>[2x]GSANDSPAKSLVDIDLSSLRDPAGIFELVEVVGNGTYGQVYKGRHVKTGQLAAIKVMDVTEDEEEEIKLEINMLKKYSHHRNIATYYGAFIKKSPPGHDDQLWLVMEFCGAGSITDLVKNTKGNTLKEDWIAYISREILRGLAHLHIHHVIHRDIKGQNVLLTENAEVKLVDFGVSAQLDREVGRRNTFIGTPYWMAPEVIACDENPDAT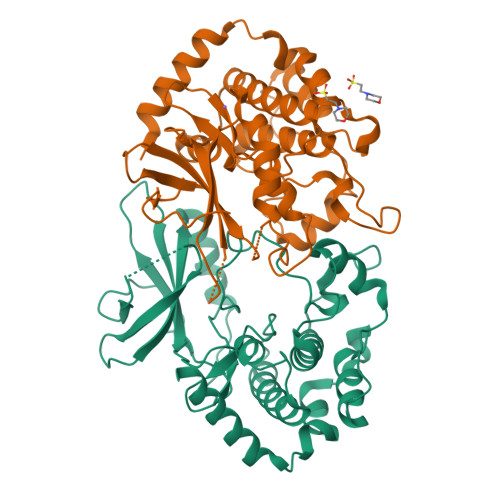YDYRSDLWSCGITAIEMAEGAPPLCDMHPMRALFLIPRNPPPRLKSKKWSKKFFSFIEGCLVKNYMQRPSTEQLLKHPFIRDQPNERQVRIQLKDHIDRTRKKRGEKDETEYEYSGSEEGNS Two of the six classes of the United States Food and Drug Administration (FDA) approved drugs for HIV-1 treatment target the reverse transcriptase (RT) protein, an enzyme critical for the replication cycle of HIV-1. While NNRTIs are allosteric inhibitors that alter the chemical catalysis rate limiting step through conformational changes, NRTIs mimic nucleotides that bind to the active site of RT. Since NRTIs lack the 3′-hydroxyl group necessary for chain elongation, their incorporation results in termination of the viral DNA transcription. In this study, we describe the crystal structures of RT in post-catalytic complexes with double stranded DNA (dsDNA) and two NRTIs —the triphosphate form of cytidine analogue (-)FTC (2′,3′-dideoxy-5-fluoro-3′-thiacytidine) and the triphosphate form of the thymidine analogue d4T (2′,3′-didehydro-2′,3′-dideoxythymidine).

Furthermore, the RT post-catalytic complex with d4T reveals the electron density of two copies of the inhibitor. One copy of d4T-MP is incorporated in the DNA primer and is flipped out of the N site by a second molecule of d4T-TP bound in the N site. Moreover, the crystal structure shows that d4T-MP is stabilized in the flipped conformation by van der Waals contacts with residue L228, which could facilitate the excision of d4T-MP from the primer. The binding mode of the d4T-MP molecule incorporated in the DNA primer is stabilized by a long-distance hydrogen bond (3.2 Å) between its 2-keto group and the side chain of residue K66. Additionally, the oxygen in the 2,5-dihydrofuran moiety is in hydrogen bond distance with a water molecule (3.0 Å). The α-phosphate group of d4T-MP is in hydrogen bond distance with the side chain of residues D110 and K220 and is making an ionic interaction with the Mg+2 ion A. Furthermore, a water molecule is bridging an interaction between the α-phosphate group of the d4T-MP incorporated in the DNA primer and the α-phosphate group of d4T-TP in the N site. In the structure of the post-catalytic complex with d4T-MP incorporated in the DNA primer the electron density for Mg+2 ion A is well defined. The Mg+2 A ion is stabilized by several hydrogen bonds with the side chains of residues D110, D185, and α-phosphate group of both bound copies of the d4T molecule. In contrast, Mg+2 ion A achieves additional coordination with the α-phosphate groups of both d4T-MP and d4T-TP in the structure of RT in post-catalytic complex with d4T-MP incorporated in the DNA primer. In fact, the α-phosphate group of d4T-TP is located ∼4 Å to the α-phosphate of d4T-MP, and the α-phosphate group of d4T-TP, acting as a nucleophile, could be attacking the α-phosphate of d4T-MP.

> MPISPIETVPVKLKPGMDGPKVKQWPLTEEKIKALVEICTEMEKEGKISKIGPENPYNTPVFAIKKKDSTKWRKLVDFRELNKRTQDFWEVQLGIPHPAGLKKKKSVTVLDVGDAYFSVPLDEDFRKYTAFTIPSINNETPGIRYQYNVLPQGWKGSPAIFQSSMTKILEPFRKQNPDIVIYQYMDDLYVGSDLEIGQHRTKIEELRQHLLRWGLTTPDKKHQKEPPFLWMGYELHPDKWTVQPIVLPEKDSWTVNDICKLVGKLNWASQIYPGIKVRQLSKLLRGTKALTEVIPLTEEAELELAENREILKEPVHGVYYDPSKDLIAEIQKQGQGQWTYQIYQEPFKNLKTGKYARMRGAHTNDVKQLTEAVQKITTESIVIWGKTPKFKLPIQKETWETWWTEYWQATWIPEWEFVNTPPLVKLWYQLEKEPIVGAETFYVDGAANRETKLGKAGYVTNRGRQKVVTLTDTTNQKTELQAIYLALQDSGLEVNIVTDSQYALGIIQAQPDQSESELVNQIIEQLIKKEKVYLAWVPAHKGIGGNEQVDKLVSAGIRKVL;> MGSSHHHHHHSSPISPIETVPVKLKPGMDGPKVKQWPLTEEKIKALVEICTEMEKEGKISKIGPENPYNTPVFAIKKKDSTKWRKLVDFRELNKRTQDFWEVQLGIPHPAGLKKKKSVTVLDVGDAYFSVPLDEDFRKYTAFTIPSINNETPGIRYQYNVLPQGWKGSPAIFQSSMTKILEPFRKQNPDIVIYQYMDDLYVGSDLEIGQHRTKIEELRQHLLRWGLTTPDKKHQKEPPFLWMGYELHPDKWTVQPIVLPEKDSWTVNDIQKLVGKLNWASQIYPGIKVRQLSKLLRGTKALTEVIPLTEEAELELAENREILKEPVHGVYYDPSKDLIAEIQKQGQGQWTYQIYQEPFKNLKTGKYARMRGAHTNDVKQLTEAVQKITTESIVIWGKTPKFKLPIQKETWETWWTEYWQATWIPEWEFVNTPPLVKLWYQLEKEPIVGAETF>IKVVRSEKEIVVLTRFEEYHFDLEKGILKDFYTMVDGRKHVFTYGNDGFDVLDEGTPLTVIEEPIVTGVGKVSEGFS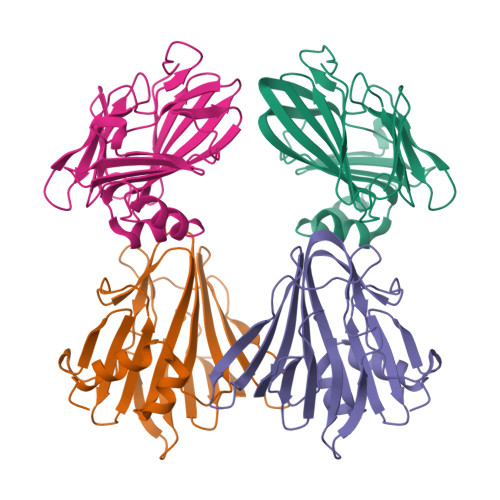DEVSMVYNYGYVKKIFTIKNNENYTFFVDIESSKPVDVTVPRVSVDTSTDRYMENYFASFNPKTRTLVLLKHDEGLLFEGTLKVNGQKRFIVFMGPNKRTLIKKAFPEDYDVLIKALVNIPGHHHHHH[4x]> MNKKYRLLFLSTPVGALGSGIGGGVELTLQNAAKALMAKGHEVEIVAPEGSVTNVTKLTPIAGNSQVSAQTQVGTDMVVLPQDSVLENMWSYAREVQDQFDLLFNFAYDWLPLYLTPFFHRPIAHWISMSSLSPVIDAMVSKTVKLCPQAIAVNTRACAD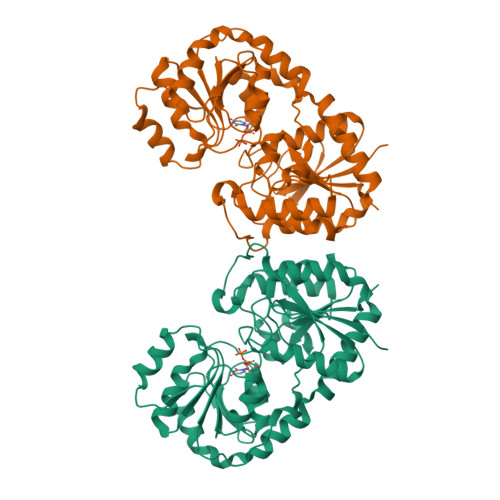TFSDGDRLMIMGKGIDVTQYNFVAKPEKPSLAWVGRISPEKGLEDAAETAQATGLPLRVFGLIQDQAYWQQIQNDFPKAEIHYEGFLSTHELQQKLGQSSALLMTPRWIEAFGNAAIEAFACGVPVISYRSGGLTEIVRHGKTGFLVDMGSVAGLIEAVSKLETIDRLACRQQLEEEYSLEVWGDRLEKWFEQLITSYTLSRNI One of the best studied adhesins is PrgB from the conjugative plasmid pCF10 of Enterococcus faecalis, which has been shown to play major roles in conjugation, biofilm formation, and importantly also in bacterial virulence. PrgB is the main adhesin produced by pCF10 and has been studied for well over three decades. This protein is around 140 kDa in size and possesses an N-terminal signal sequence and a C-terminal LPXTG cell wall anchor motif. PrgB, which is indicated to function as a dimer in vivo, distributes over the entire surface of the cell wall and increases cellular aggregation, biofilm formation, and the efficiency of plasmid transfer. PrgB seems to consist of an N-terminal disordered region (residues 35–197), followed by a newly identified coiled-coil (COI) domain (residues 198–257), the previously crystallized polymer adhesin domain (residues 261–558), a linker region (residues 559–582), four immunoglobulin (Ig)-like domains (residues 583–1232), and finally the C-terminal disordered region containing the LPXTG motif (residues 1263–1305) that gets anchored to the cell wall.

Crystals belonging to space group P212121 appeared after 8–12 weeks, diffracted to 1.85 Å and contained two molecules in the asymmetric unit. Surprisingly, the resulting electron density lacked the previously crystallized polymer adhesin domain of PrgB, and instead only contained residues 584–1233. There is also no space in the crystal packing to allow for a flexible polymer adhesin domain, so it was likely cleaved off in the crystallization drop before the crystals were formed. The modeled protein indeed consists of four Ig-like domains: two CSA and two CSC domains. The Ig-like domains seem to come in pairs of two slightly different structures, denoted as CSA1–CSC1 (first pair) and CSA2–CSC2 (second pair), as named in InterPro (CSA from IPR026345; adhesin isopeptide-forming adherence domain, and CSC from IPR032300; cell-surface antigen C-terminal). In each of the Ig-like domains of PrgB, isopeptide bonds are formed between a lysine and an asparagine, a bond which is further stabilized by an aspartic acid. There is density in the conserved metal-binding site of the CSA2 domain that has been suggested to bind Ca2+ in the Antigen I/II proteins. Refinement of our structure indicated that Mg2+ was the best fit to the density. The homologous C2 domains from AspA, Pas, SpaP, and SspB, each have an extra structural feature termed the BAR (SspB adherence region) domain, which mediates adherence in these proteins. This BAR domain is absent in PrgB. The structure that we determined shows that these two sequence motifs are not surface exposed, but instead play an important role in the structural integrity of the interfaces between CSA1 and CSC1, and between CSA2 and CSC2.

>[2x]PVLVPNKEVTDGQKNINDLNVKRGDSLQYIVTGDTTELAKVDPKTVTKQGIRDTFDAEKVTIDLSKVKVYQADASLNEKDLKAVAAAINSGKAKDVTASYDLNLDQNTVTAMMKTNADGSVVLAMGYKYLLVLPFVVKNVEGDFENTAVQLTNDGETVTNTVINHVPSSNPSKDVKADKNGTVGSVSLHDKDIPLQTKIYYEVKSSERPANYGGITEEWGMNDVLDTTHDRFTGKWHAITNYDLKVGDKTLKAGTDISAYILLENKDNKDLTFTMNQALLAALNEGSNKVGKQAWSVYLEVERIKTGDVENTQTENYNKELVRSNTVVTHTPDDPKPTKAVHNKKGEDINHGKVARGDVLSYEMTWDLKGYDKDFAFDTVDLATGVSFFDDYDETKVTPIKDLLRVKDSKGVDITNQFTISWDDAKGTVTISAKDPQAFILAYGGQELRVTLPTKVKADVSGDVYNSAEQNTFGQRIKTNTVVNHIPKVNPKKDVVIKVGDKQSQNGATIKLGEKFFYEFTSSDIPAEYAGVVEEWSISDKLDVKHDKFSGQWSVFANSNFVLADGTKVNKGDDISKLFTMTFDKGVVKITASQAFLDAMNLKENKNVAHSWKAFIGVERIAAGDVYNTIEESFNNEKIKTNTVVTHTPE[3,4-bis(fluoranyl)phenyl]-(4-methylpiperazin-1-yl)methanone 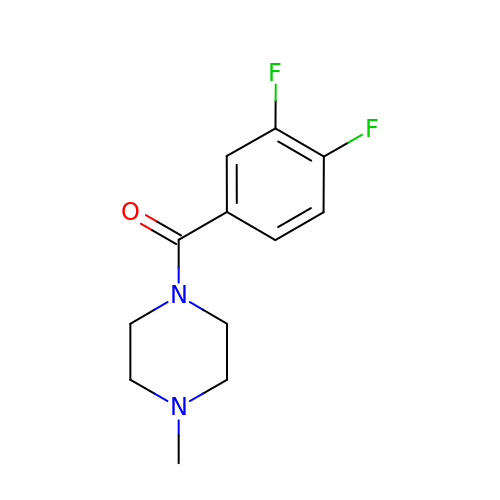| C12 H14 F2 N2 O | ZCPNSVBDWJVJSY-UHFFFAOYSA-N> GQPNSFTNQCPGETCVIPNDDTLVGRADEKVNERHSPQTEPMITSIGNPAQVLKVKETFGTWLRESANRSDDRIWVTEHFSGIMVKEFEDLPALLNSSFTLLHLPHYFHGCGHAVYN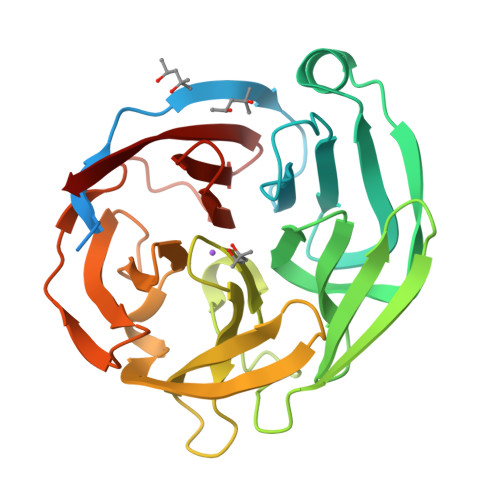NSLYYHKGGSNTIVRFEFGKETPQTLKLEDALYFDRKYLFANSKTYFNIAVDEKGLWIIYASSVDGSSILVAQLDERTFSVLRHINTTYPKSKAGNAFIAQGILYVTDTKDTRVTFAFDLLRGKQINANFGLRMSQSVLAMLSYNMRDQHLYSWEDGHLMLYPVHFSS>GTVTTDGADIVIKTKGGLEVATTDKEFSFKLGGRLQADYGRFDGYYTNNGNTADAAYFRRAYLEFGGTAYRDWKYQINYDLSRNVGNDSAGYFDEASVTYTGFNPVNLKFGRFYTDFGLEKATSSKWVTALERNLTYDIADWVNDNVGTGIQASSVVGGMAFLSGSVFSENNNDTDGDSVKRYNLRGVFAPLHEPGNVVHLGLQYAYRDLEDSAVDTRIRPRMGMRGVSTNGGNDAGSNGNRGLFGGSSAVEGLWKDDSVWGLEGAWALGAFSAQAEYLRRTVK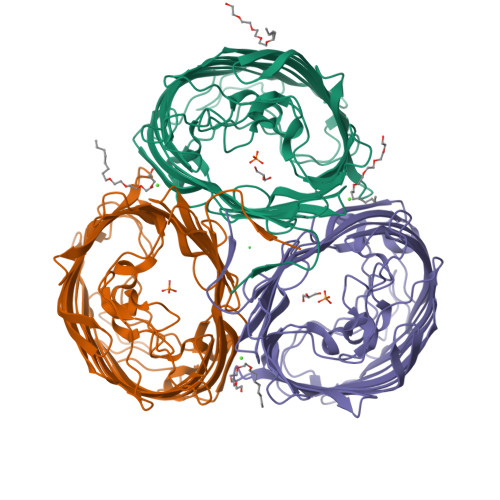AERDREDLKASGYYAQLAYTLTGEPRLYKLDGAKFDTIKPENKEIGAWELFYRYDSIKVEDDNIVVDSATREVGDAKGKTHTLGVNWYANEAVKVSANYVKAKTDKISNANGDDSGDGLVMRLQYVF[3x]>[40x]MLYL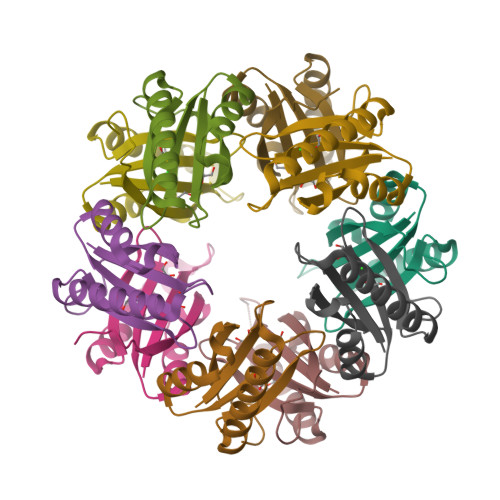VRMTVNLPRNLDPREEERLKASEKARSRTLQEQGQWRYLWRTTGKYGNISVFDVNSHDELHEILWSLPFFPYLTIDVEPLSHHPARVGKD>HHHHHHMAPERLRSTILTKDGINWYYEQEGSGPDVVLIPDGLGDCQMFDKPMSIIGSSGFKVTTFDMPGMSRSSSAPPETYQDVTGQKLANYIVTVMDQLGIKTASVWGCSSGASTVLALCSGFPERVRNGMPHEVPTANPENLQNIHDADPATISRDMAAVSRAMSANEEAWDALGPEVHERLRDNYVRWAYGYPRTIPGSAATKTEDLHKVPIDWTVGAAGPTQVFFENVVIATRESIPIKTLPGFHFPYVSHPEAFAKYVV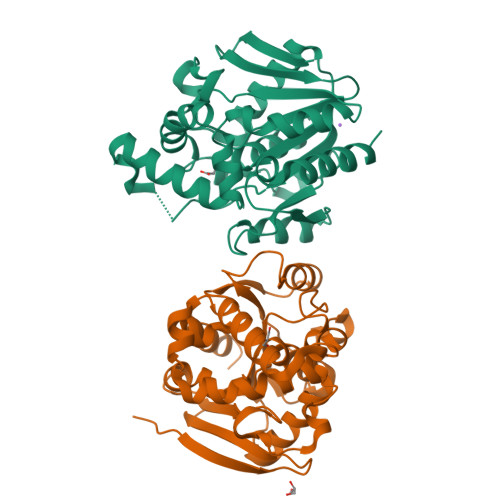ETTRKYL[4x]>MGGPVEILPFLYLGSAYHAARRDMLDALGITALLNVSSDCPNHFEGH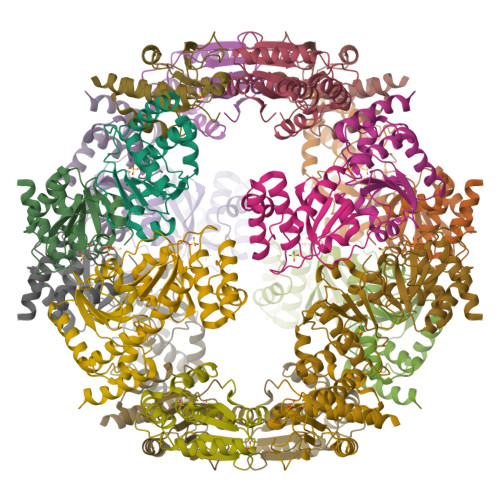YQYKCIPVEDNHKADISSWFMEAIEYIDAVKDCRGRVLVHSQAGISRSATICLAYLMMKKRVRLEEAFEFVKQRRSIISPNFSFMGQLLQFESQVLA[6x]>QTNWLAEIVECDRVSSNVVRLLLQPLTADGAAPISLNFAPGQFVDIEIPGTHTRRSYSMASVAEDGRLEFFIRLLPDGAF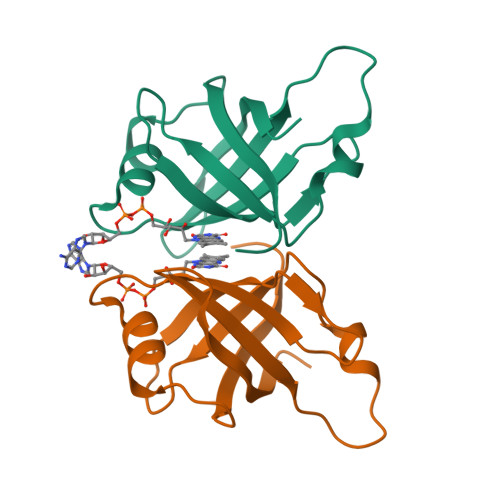SNYLRTQASVGQRVALRGPAGSF[2x]>[2x]MVYQVK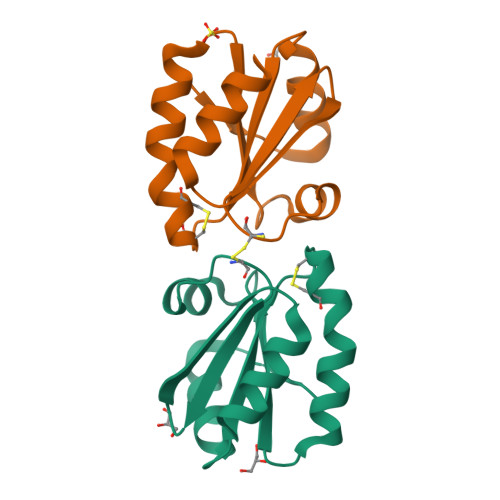DQEDFTKQLNEAGNKLVVIDFYATWCGPCKMIAPKLEELSQSMSDVVFLKVDVDECEDIAQDNQIACMPTFLFMKNGQKLDSLSGANYDKLLELVEKNK>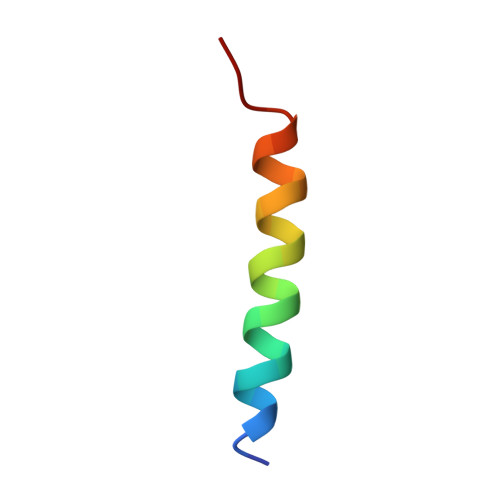 NHAIYEKAKEVSSALSKVLSKIDDT>[2x]SVKSEYAEAAAVGQEAVAVFNTMKAAFQNGDKEAVAQYL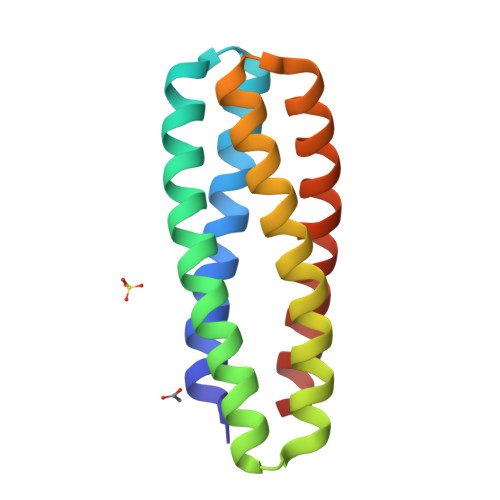ARLASLYTRHEELLNRILEKARREGNKEAVTLMNEFTATFQTGKSIFNAMVAAFKNGDDDSFESYLQALEKVTAKGETLADQIAKAL> MDVVDIARWQFGITTVYHFIFVPLTIGLAPLVAIMQTFWQVTGKEHWYRATRFFGTVLLINFAVGVATGIVQEFQFGMNWSEYSRFVGDVFGGPLALEGLIAFFLESVFLGLWIFGWGKIPGWLHTASIWIVAIATNISAYFIIVANSFMQHPVGAEYNPETGRAELTDFWALLTNSTALAAFPHAVAGGFLTAGTFVLGISGWWIIRAHRQAKKAEAEIESKHSMHRPALWVGWWTTVVSSVALFITGDTQAKLMFVQQPMKMASAESLCETATDPNFSILTIGTHNNCDTVTHLIDVPFVLPFLAEGKFTGVTLQGVNQLQAAAEQAYGPGNYSPNLFVTYWSFRAMIGLMLGSLAIAAIAWLLLRKKRTPTGKIARLFQIGSLIAIPFPFLANSAGWIFTEMGRQPWVVHPNPESAGDARTEMIRMTVDMGVSDHAPWQVWLTLIGFTILYLILFVVWVWLIRRAVLIGPPEEGAPSVEAKTGPATPIGSDMPMTPLQFTAAAPTTREKE;> MDHNTFWFILIAFLFSGYF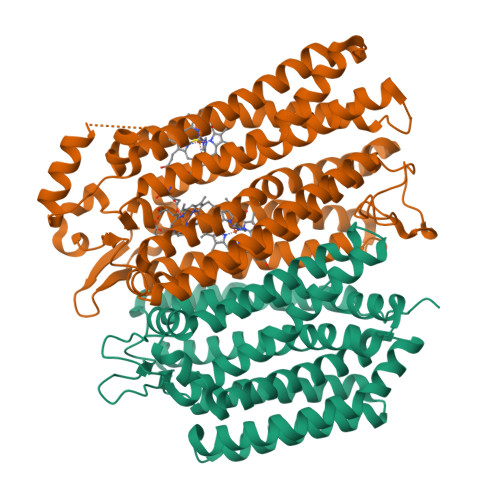LLEGFDFGVGILAPIIGKDSAARNTVIRTIGPVWDGNEVWLIVAGGALFAAFPEWYATMFSGMYLPLFLVLVSLIIRVVGLEWRKKVDDPRWQKWSDRAIFIGSWTPPLMWGFIFANILRGMPIKADHTIDAAAALPGMVNVFAILGALAFTALFALHGLAFIRLKTAGRVRTDAAKAAPGVALLAAVTGGPFVLWAAIAYGRSWSWILAVLIIAAVLGGAFALIKDRDGLSFLSTSVAVIGVVALLFSSLFPNVMPTTLADGVSLDIWNASASHYALTILTWTAAVIAPLVVLYQGWTYWVFRKRLHAEPVSA> TYNGCSSSEQSALAAAASAAQSYVAESLSYLQTHTAATPRYTTWFGSYISSRHSTVLQHYTDMNSNDFSSYSFDCTCTAAGTFAYVYPNRFGTVYLCGAFWKAPTTGTDSQAGTLVHESSHFTRNGGTKDYAYGQAAAKSLATMDPDKAVMNADNHEYFSENNPAQ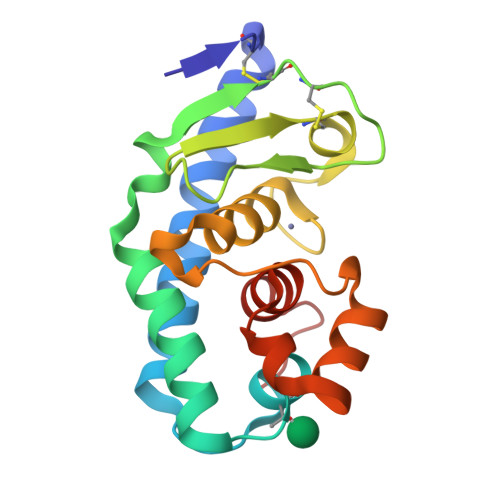S>[2x]MGSSHHHHHHSSGRENLYFQGMPKLILASTSPWRRALLEKLQISFECAAPEVDETPRSDESPRQLVLRLAQEKAQSLASRYPDHLIIGSDQVCVLDGEITGKPLTEENARLQLRKASGNIVTFYTGLALFNSANGHLQTEVEPFDVHFRHLSEAEIDNYVRKEHPLHCAGSFKSEGFGITLFERLEGRDPNTLVGLPLIALCQMLRREGKNPLMG

Maf (for multicopy associated filamentation) proteins represent a large family of conserved proteins implicated in cell division arrest but whose biochemical activity remains unknown. Here, we show that the prokaryotic and eukaryotic Maf proteins exhibit nucleotide pyrophosphatase activity against 5-methyl-UTP, pseudo-UTP, 5-methyl-CTP, and 7-methyl-GTP, which represent the most abundant modified bases in all organisms, as well as against canonical nucleotides dTTP, UTP, and CTP. The protomer structures of the four Maf proteins revealed a large β sheet containing seven β strands (β1 to β7) with two α-helical subdomains on one side and one long α helix on another side. Thus, pyrophosphatase activity of Maf proteins toward canonical and modified nucleotides might provide the molecular mechanism for a dual role of these proteins in cell division arrest and house cleaning.

Screening of Maf proteins for pyrophosphatase activity against a set of 57 noncanonical or modified nucleoside triphosphates revealed that the YhdE-like Maf proteins (E. coli YhdE, BSU28050, YOR111W, and ASMTL-Maf) also exhibited high pyrophosphatase activity against 5-methyl-UTP (m5UTP or riboTTP), pseudouridine triphosphate (pseudo-UTP or Ψ), and 5-methyl-CTP (m5CTP), whereas the two YceF proteins (from E. coli and S. typhimurium) were active toward 7-methyl-GTP (m7GTP). The Michaelis-Menten constant, KM, of the YhdE-like proteins toward canonical pyrimidine nucleotides varied in a micromolar range: 32.7–53.0 μM for dTTP; 29.7–72.4 μM for UTP; and it was lower (to a lesser extent for ASMTL-Maf) with modified nucleotides (4.7–47.2 μM). Both YceF proteins also showed high affinity to m7GTP (32.8 μM for YceF and 30.9 μM for STM1189). Hydrolysis of m7GTP by the E. coli YceF was inhibited in a dose-dependent manner by unmodified nucleotides, with 50% reduction at 80–100 μM (GTP, ATP, UTP), which is higher than its KM to m7GTP (32.8 μM). The two structures of YceF-like Maf proteins (Tb-Maf1 and YceF) appear to display an open conformation of the active site, which can accommodate a nucleoside group of the substrate without any conformational change in the binding pocket. The Tb-Maf1 contains a phenylalanine residue at this site (Phe16) whose side chain points away from the pocket, whereas the Glu170 side chain is oriented toward the pocket and can participate in base recognition. This Glu residue is conserved in YceF (Glu154) and other YceF-like Maf proteins, making it the signature residue-3 of the YceF subfamily motif. In the YceF structure, the Glu154 side chain is partly disordered, suggesting local structural flexibility. It should be noted that the YceF E154A mutant protein retained the wild-type level of substrate affinity and catalytic activity. The Tb-Maf1 Gln86 (Gln70 in YceF) resides at the bottom of the pocket, providing the side chain-main chain H-bonds to the C end of the α6 helix and thus determining the size of the guanine recognition site.> MGHHHHHHHHHSSG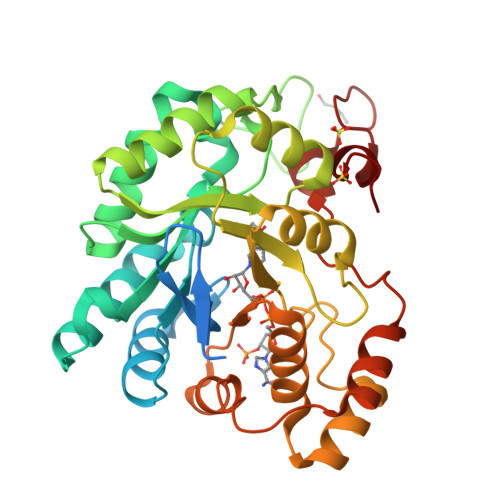HIDDDDKHMLEASAKATMGQGEQDHFVLKSGHAMPAVGLGTWRAGSDTAHSVRTAITEAGYRHVDTAAEYGVEKEVGKGLKAAMEAGIDRKDLFVTSKIWCTNLAPERVRPALENTLKDLQLDYIDLYHIHWPFRLKDGAHMPPEAGEVLEFDMEGVWKEMENLVKDGLVKDIGVCNYTVTKLNRLLRSAKIPPAVCQMEMHPGWKNDKIFEACKKHGIHITAYSPLGSSEKNLAHDPVVEKVANKLNKTPGQVLIKWALQRGTSVIPKSSKDERIKENIQVFGWEIPEEDFKVLCSIKDEKRVLTGEELFVNKTHGPYRSARDVWDHEN(2Z,4E)-2,6-dihydroxyhexa-2,4-dienoic acid | C6 H8 O4 | 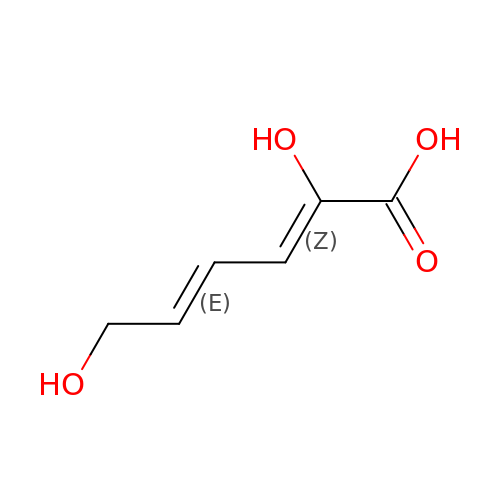YRYDCWGBHNTXLE-WFTYEQLWSA-N> MVQRWLYSTNAKDIAVLYFMLAIFSGMAGTAMSLIIRLELAAPGSQYLHGNSQLFNVLVVGHAVLMIFFLVMPALIGGFGNYLLPLMIGATDTAFPRINNIAFWVLPMGLVCLVTSTLVESGAGTGWTVYPPLSSIQAHSGPSVDLAIFALHLTSISSLLGAINFIVTTLNMRTNGMTMHKLPLFVWSIFITAFLLLLSLPVLSAGITMLLLDRNFNTSFFEVSGGGDPILYEHLFWFFGHPEVYILIIPGFGIISHV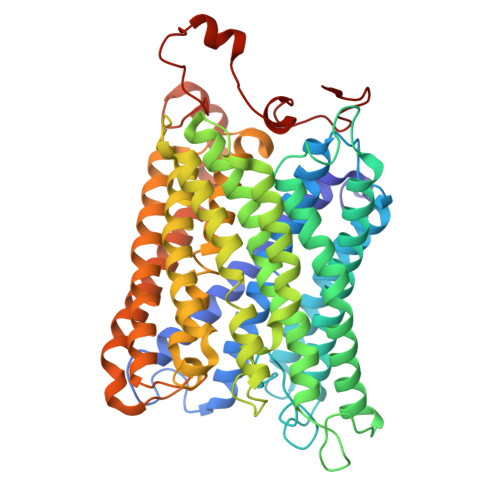VSTYSKKPVFGEISMVYAMASIGLLGFLVWSHHMYIVGLDADTRAYFTSATMIIAIPTGIKIFSWLATIHGGSIRLATPMLYAIAFLFLFTMGGLTGVALANASLDVAFHDTYYVVGHFHYVLSMGAIFSLFAGYYYWSPQILGLNYNEKLAQIQFWLIFIGANVIFFPMHFLGINGMPRRIPDYPDAFAGWNYVASIGSFIATLSLFLFIYILYDQLVNGLNNKVNNKSVIYNKAPDFVESNTIFNLNTVKSSSIEFLLTSPPAVHSFNTPAVQS>MQEGKVKWFNNEKGYGFIEVEGGSDVFVHFTAIQGEGFKTLE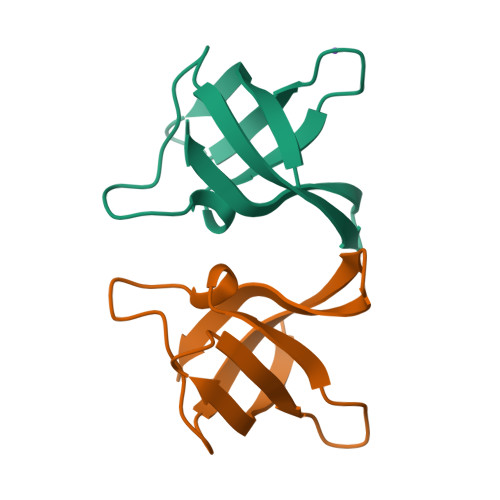EGQAVSFEIVQGNRGPQAANVVKE[2x]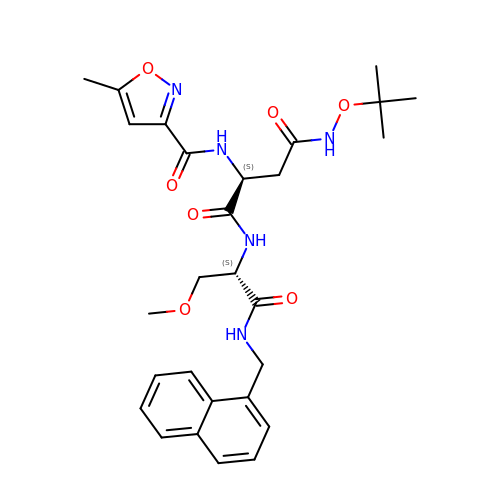N-tert-butoxy-N~2~-(5-methyl-1,2-oxazole-3-carbonyl)-L-asparaginyl-O-methyl-N-[(naphthalen-1-yl)methyl]-L-serinamide | C28 H35 N5 O7 | SDQPNMCIUPBBDV-GMAHTHKFSA-N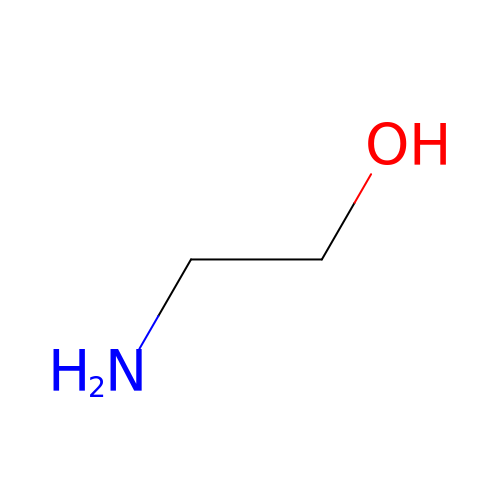ETHANOLAMINE | C2 H7 N O | HZAXFHJVJLSVMW-UHFFFAOYSA-N> MNVTPLDELQWKSPEWIQVFGLRTENVLDYFAESPFFDKTSNNQVIKMQRQFSQLNDPNAAVNMTQNIMTLPDGKNGNLEEEFAYVDPARRQILFKYPMYMQLEEELMKLDGTEYVLSSVREPDFWVIRKQRRTNNSGVGSAKGPEIIPLQDYYIIGANIYQSPTIFKIVQSRLMSTSYHLNSTLESLYDLIEFQPSQGVHYKVPTDTSTTATAATNGNNAGGGSNKSSVRPTGGANMATVPSTTNVNMTVNTMGTGGQTIDNGTGRTGNGNMGITTEMLDKLMVTSIRST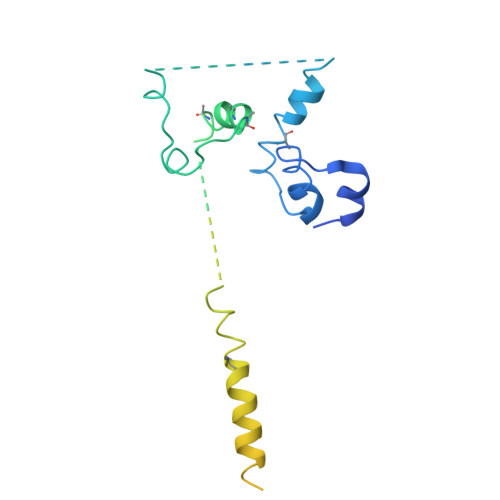PNYI> YIFSKLCTFTITQKEFMNQHWYHCHTCKMVDGVGVCTVCAKVCHKDHEISYAKYGSFFCDCGAKEDGSCLALVK

The N-end rule pathway is a proteolytic system involving the destabilization of N-terminal amino acids, known as N-degrons, which are recognized by N-recognins. The E3 ligases of the UBR subfamily recognize and degrade N-degrons through the ubiquitin-proteasome system. However, unlike other UBR proteins, UBR4, despite having only the UBR box domain, can recognize both type-1 and type-2 N-degron. Our findings suggest that the UBR box of UBR4 recognizes type-1 N-terminal arginine and type-2 N-terminal amino acids containing an aromatic ring, such as tyrosine, tryptophan, and phenylalanine through pi-interaction with two phenylalanines of the UBR box of UBR4.

Therefore, we attempted to determine the structure of UBR4UBR in complex with YIFS to investigate how the distinctive feature of UBR4UBR observed in its apo structure affects ligand binding and how UBR4UBR can recognize type-2 N-degrons. To overcome this issue, we purified the protein with the N-terminus starting with tyrosine (YIFS-UBR4UBR) using the LC3B tag system. Using this system we successfully established the crystal structure of YIFS-UBR4UBR. We found that the N-terminal residue of one YIFS-UBR4UBR molecule binds to the ligand-binding site of another. As expected, the first amino group of YIFS-UBR4UBR was bound to the carboxyl group of Asp1715 and the oxygen atom of Phe1713, as in the other UBR boxes. However, unlike the structure of the arginine-bound UBR box of UBR1 and UBR2, the direction of the N-terminal tyrosine residue was not toward Asp1721, but toward Phe1671 and Phe1713 in the binding site. These two phenylalanine residues on the ligand-binding surface of UBR4UBR create a hydrophobic patch, which explains the binding ability of residues with aromatic rings. Between Phe1671 and Phe1713 of the YIFS-UBR4UBR and Tyr1 of the ligand form trimeric pi–pi interactions, and Phe1671 and Phe3 of the ligand form typical T-shaped pi–pi interaction. In these pi–pi interactions, the distances (Rcen) fall within the range of 4.7 to 6.5 Å, which is the typical distance range for the pi–pi interaction. The presence of pi–pi interactions can greatly enhance the preference for amino acids containing aromatic rings, such as tyrosine.>[2x]MAHHHHHHVGTSFRGKNAVVTGGAGGIGLQVSKQLLAAGAAKVAIIDLQDNLEEFVKLRAAHPTQSVMIIKMDVANKKGVEATYEEIAKTFGNIDIVVNVAGIFNDKDVQRTLLVNLGGIINSTLSALPYMGKDNGGKGGIVVNMSSVVGLDPMFIIPVYGATKAGIINFTRCLANEKYYQRSGIKFVTVCPGATMTDMFTNFTEKIIFPETSDET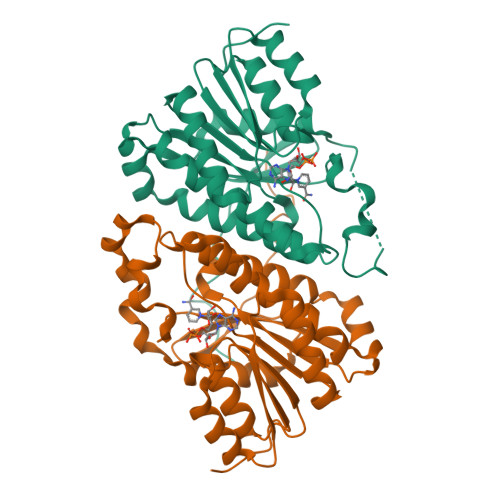YRILDRLNKQSAADVSRCILNVLEKDKNGAVYVIEGKRVYPLEIKPQWTGKEQAL> SRNICYDAFVSYSERDAYWVENLMVQELENFNPPFKLCLHKRDFIPGKWIIDNIIDSIEKSHKTVFVLSENFVKSEWCKYELDFSHFRL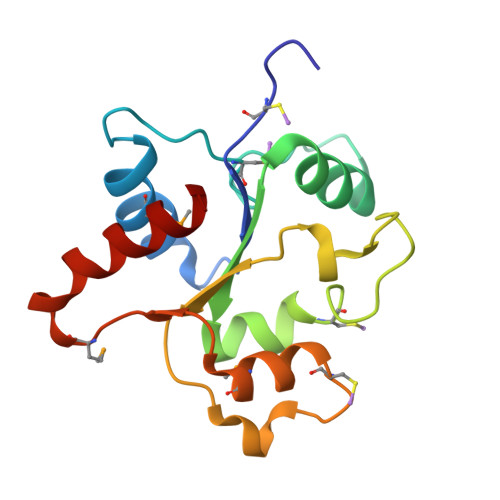FDENNDAAILILLEPIEKKAIPQRFCKLRKIMNTKTYLEWPMDEAQREGFWVNLRAAIKS> MNVGTAHSEVNPNTRVMNSRGIWLSYVLAIGLLHIVLLSIPFVSVPVVWTLTNLIHNMGMYIFLHTVKGTPFETPDQGKARLLTHWEQMDYGVQFTASRKFLTITPIVLYFLTSFYTKYDQIHFVLNTVSLMSVLIPKLPQLHGVRIFGINKY;>[2x]MATATEQWVLVEMVQALYEAPAYHLILEGILILWIIRLLFSKTYKLQERSDLTVKEKEELIEEWQPEPLVPPVPKDHPALNYNIVSGPPSHKTVVNGKECINFASFNFLGLLDNPRVKAAALASLKKYGVGTCGPRGFYGTFDVHLDLEDRLAKFMKTEEAIIYSYGFATIASAIPAYSKRGDIVFVDRAACFAIQKGLQASRSDIKLFKHNDMADLERLLKEQEIEDQKNPRKARVTRRFIVVEGLYMNTGTICPLPELVKLKYKYKARIFLEESLSFGVLGEHGRGVTEHYGINIDDIDLISANMENALASIGGFCCGRSFVIDHQRLSGQGYCFSASLPPLLAAAAIEALNIMEENPGIFAVLKEKCGQIHKALQGISGLKVVGESLSPAFHLQLEESTGSREQDVRLLQEIVDQCMNRSIALTQARYLEKEEKCLPPPSIRVVVTVEQTEEELERAASTIKEVAQAVLL;> MADYKDDDDKSGPDEVDASGRMAGMALARAWKQMSWFYYQYLLVTALYMLEPWERTVFNSMLVSIVGMALYTGYVFMPQHIMAILHYFEIVQ;> MRPEPGGCCCRRTVRANGCVANGEVRNGYVRSSAAAAAAAAAGQIHHVTQNGGLYKRPFNEAFEETPMLVAVLTYVGYGVLTLFGYLRDFLRYWRIEKCHHATEREEQKDFVSLYQDFENFYTRNLYMRIRDNWNRPICSVPGARVDIMERQSHDYNWSFKYTGNIIKGVINMGSYNYLGFARNTGSCQEAAAKV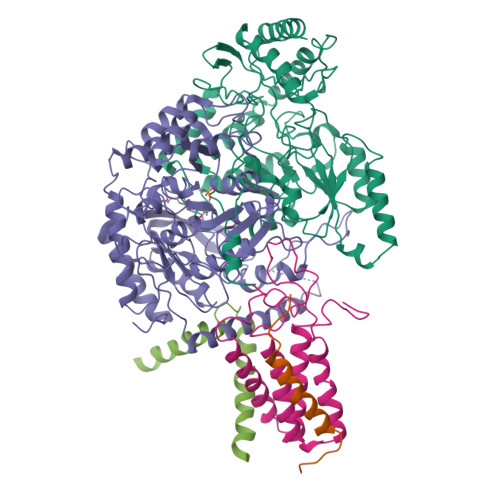LEEYGAGVCSTRQEIGNLDKHEELEELVARFLGVEAAMAYGMGFATNSMNIPALVGKGCLILSDELNHASLVLGARLSGATIRIFKHNNMQSLEKLLKDAIVYGQPRTRRPWKKILILVEGIYSMEGSIVRLPEVIALKKKYKAYLYLDEAHSIGALGPTGRGVVEYFGLDPEDVDVMMGTFTKSFGASGGYIGGKKELIDYLRTHSHSAVYATSLSPPVVEQIITSMKCIMGQDGTSLGKECVQQLAENTRYFRRRLKEMGFIIYGNEDSPVVPLMLYMPAKIGAFGREMLKRNIGVVVVGFPATPIIESRARFCLSAAHTKEILDTALKEIDEVGDLLQLKYSRHRLVPLLDRPFDETTYEETED> AGATGCACTGCTGT;> CGGACAGCAGTGCAT;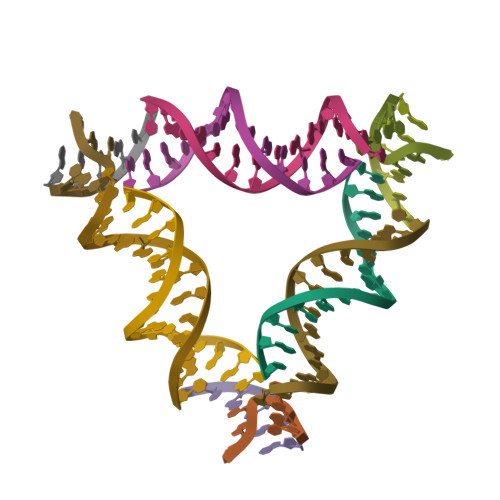> CACCCGT;> CTGTGA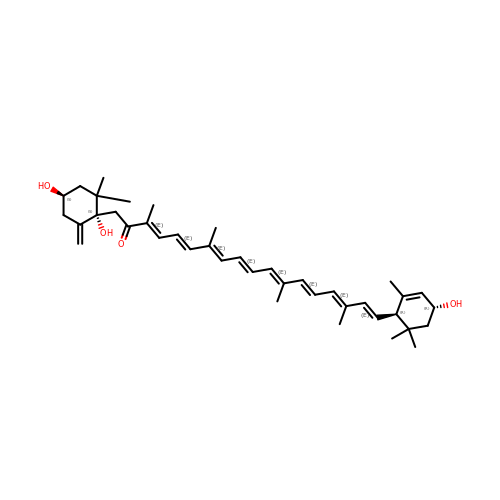(3~{E},5~{E},7~{E},9~{E},11~{E},13~{E},15~{E},17~{E})-1-[(1~{S},4~{S})-2,2-dimethyl-6-methylidene-1,4-bis(oxidanyl)cyclohexyl]-3,7,12,16-tetramethyl-18-[(1~{R},4~{R})-2,6,6-trimethyl-4-oxidanyl-cyclohex-2-en-1-yl]octadeca-3,5,7,9,11,13,15,17-octaen-2-one | C40 H56 O4 | WOJYJHBMWRNRJG-ITGJSFTBSA-N6-amino-4-phenyl-1,3,5-triazin-2(1H)-one | C9 H8 N4 O | 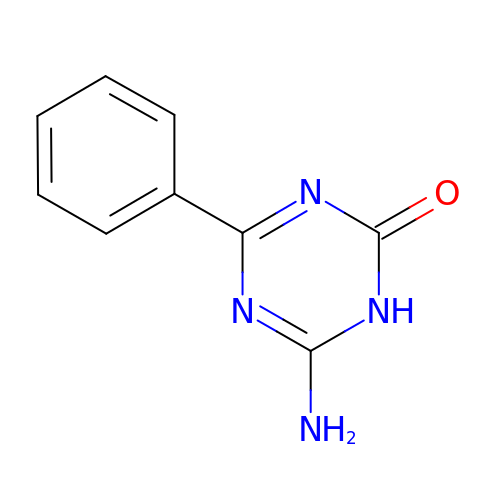ZBKCUYOBOGCDKC-UHFFFAOYSA-N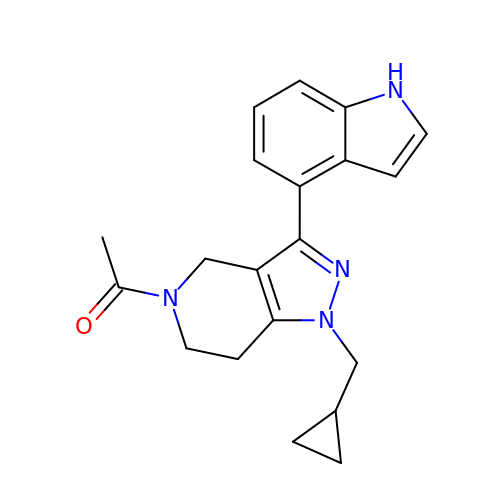1-[1-(cyclopropylmethyl)-3-(1H-indol-4-yl)-1,4,6,7-tetrahydro-5H-pyrazolo[4,3-c]pyridin-5-yl]ethan-1-one | C20 H22 N4 O | MPXKOIKIRQBXKT-UHFFFAOYSA-N> GPGSMKASWRQVFAWRMQRQFLEPRTQPSASDVVGRLCGVQAQVWSVAELNVALRQAAPDRESVNREVADLSLMKTWAMRGTLHLLRPSEAGP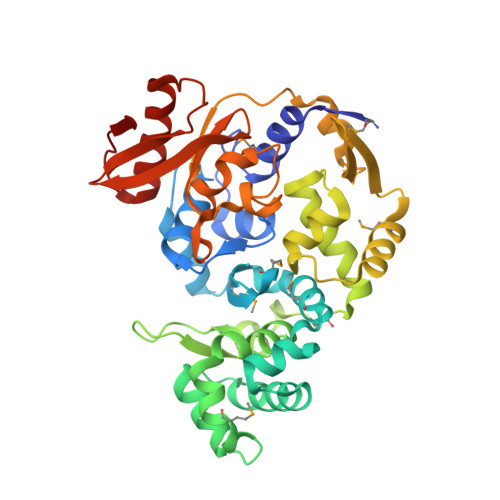YLSLMANTGSWLKPSWTRASGVTPRQVDELTEEVAGILDGVVLTRDELVTRLVADKRFVSMEERLRSGWGSVLKPLAWRGVLCHGPNRGNKITFTLPASQFGADWGKMPEPDEAAPTVIKAYLGAYGPATIETFDRWLSLNSTSKPKLRKWFGDMGDELTEVDVEGRKAFVLTEHAEELAATAPCTGIRLLGGFDQYLLGPGTKDEVVLAPEHRSAVSRAAGWISPVVVKDGRVVGVWEIVDQELVVTPFPDTERLPVKAVEKEAAHVARASGVSRLPVRIV phenanthren-9-ylacetaldehyde | C16 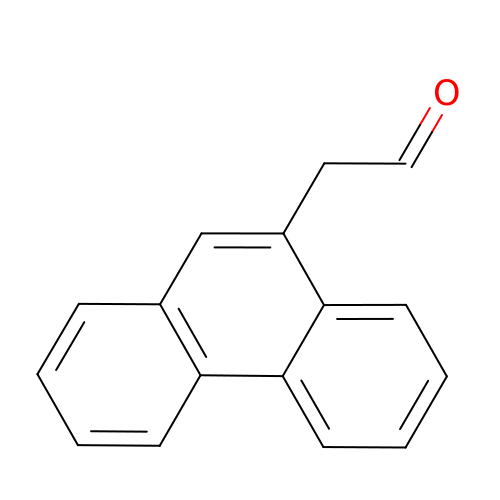H12 O | GLWZSGUBBSQBKG-UHFFFAOYSA-N>[2x]SNAQSATSEQIVDIADASFAPVIEQYRIPGLVVGITWQGQHSFYATGVAARKGNVAATPDTIFELGSISKIFTATLAALAEDRGMLDLDAPVSDSIPQLEGAAFGAIRLVDLSTHVTGGLPLQVPGEVGNVAELIRWLESWQPPQPGTRSYSNVSIGL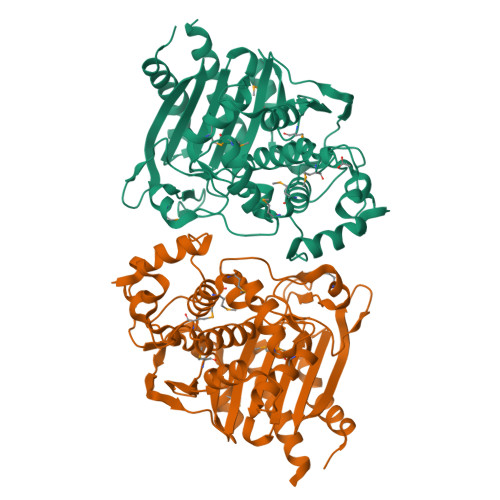LGHITAQTMGMSFAQAAQDVLFPAMGLGSTYVDVPDDAMDRYAFGYDRKTDAPIRVNPGVLADEAYGVKSTARDMLRLLDLELGRGGANPALTAALERTRQGQAETAYYTQDMIWEQYPWPVDVARMEAGNGYDFILSPQPATRLTPPLPPQRDVILNKTGATNGFGGYVALLPGQDLGIVVLANRNYPNEARVRATHALITDLLATQD>MRTRSTISTPNGITWYYEQEGTGPDIVLVPDGLGECQMFDSSVSQIAAQGFRVTTFDMPGMSRSAKAPAETYTEVTAQKLASYVISILDALDIKHATVWGCSSGASTVVALLLGYPDRIRNAMCHELPTKLLDHLSNTAVLEDEEISNILANVMLNDVSG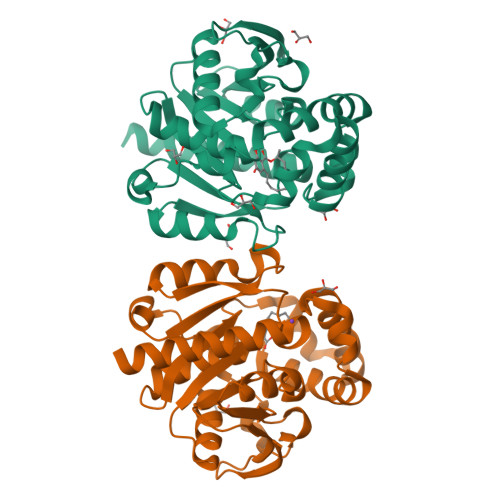GSEAWQALGVEVHARLHKNYPVFARGYPRTIPPSAPVQDVEALRGKPLDWTVGAATPTESFFDNIVTATKAGVNIGLLPGMHFPYVSHPDVFAKYVVETTQKHLWNSSSVDKLAAALEHHHHHH[2x]> SDHHHHHHGPISPIETVPVKLKPGMDGPKVKQWPLTEEKIKALVEICTEMEKEGKISKIGPENPYNTPVFAIKKKDSTKWRKLVDFRELNKRTQDFWEVQLGIPHPAGLKKKKSVTVLDVGDAYFSVPLDEDFRKYTAFTIPSINNETPGIRYQYNVLPQGWKGSPAIFQSSMTKILEPFKKQNPDIVIYQYMDDLYVGSDLEIGQHRTKIEELRQHLL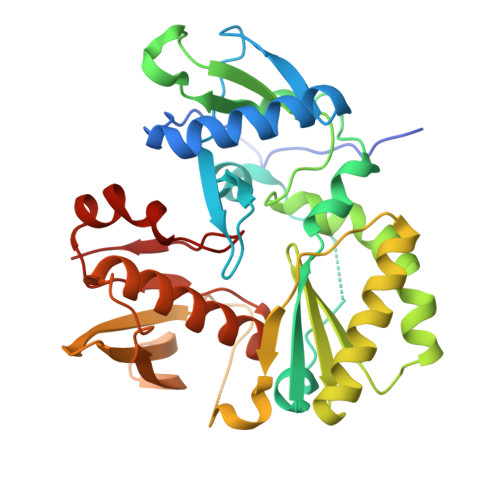RWGLTTPDGYELHPDKWTGSGSGGYDPSKDLIAEIQKQGQGQWTYQIYQEPSKNLKTGKYARKRGAHTNDVKQLTEAVQKITTESIVIWGKTPKFKLPIQKETWETWWTEYWQATWIPEWEFVN1,2,4-TRIAZOLE | C2 H3 N3 | 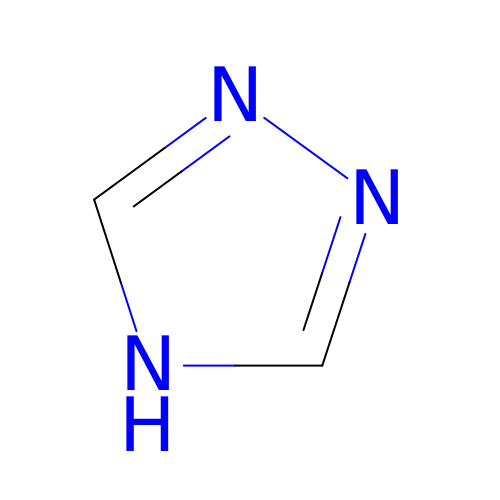NSPMIYGKQJPBQR-UHFFFAOYSA-N>[2x]EQACDICRLKKLKCSKEKPKCAKCLKNNWECRYSPKTKRSPLTRAHL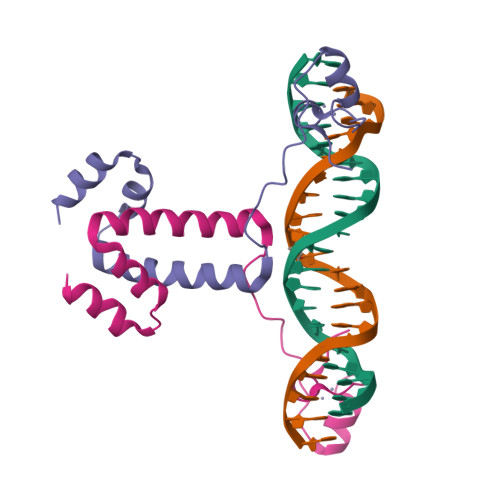TEVESRLERLEQLFLLIFPREDLDMILKMDSLQDIKALLTGL>MDGSGKAPGSEGGSAPDGALTLGFAQVGAESGWRTANTESIKSAAEEAGVNLKFADANGEQEKQISAIRSFIQQGVDVIAFSPVVRTGWDAVLQETKNAGIPVIL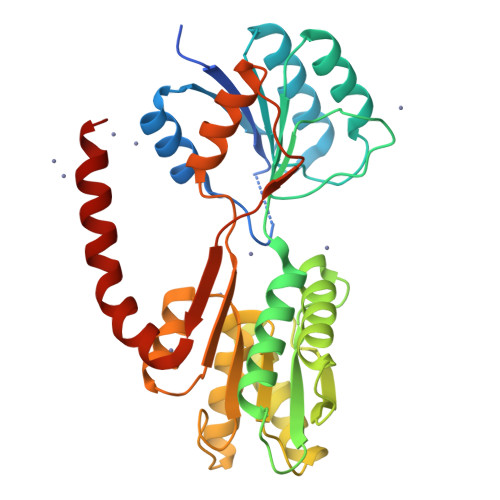TDRAVDTQDTDVYKTFIGADFIEEGRRAGQWVADQYASATGPVNIVQLEGTTGADPAIDRKTGFAEGISKNPNLKIVASQTGDFTRSGGKQVMEAFLKSTPQIDVVFAQNDDMGLGAMEAIEAAGKKPGTDIKIVAVDATHDGMQALADGKFNYIVECNPLLGPELMDLAKKVAAGEPVPERVVTPDEAFDQAQAKAALPNRQYKLAAALEHHHHHH[2x]> GSHMTSPFKLPDESPSWTEWRLHNDETNSNQDNPLGFKESWGFGKVVFKRYLRYDRTEASLHRVLGSWTGDSVNYAASRFFG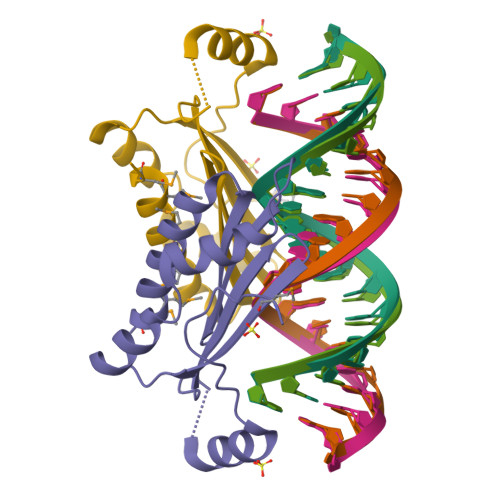FDQIGCTYSIRFRGVSITVSGGSRTLQHLCEMAIRSKQEMLQMAPIEVESNVSR3-(6-{[4-(trifluoromethoxy)phenyl]amino}pyrimidin-4-yl)benzamide | C18 H13 F3 N4 O2 | 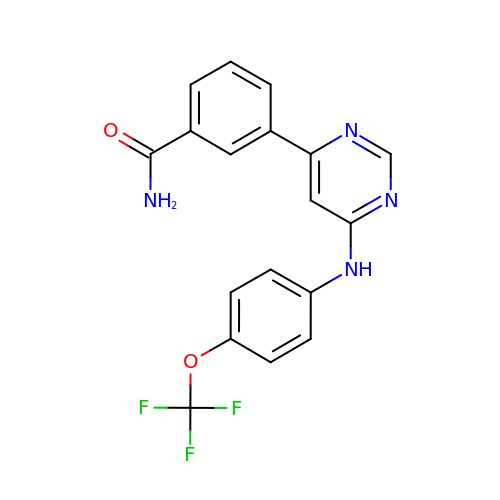WEVYNIUIFUYDGI-UHFFFAOYSA-N2-ethenyl-1-methylpyridinium | C8 H10 N | 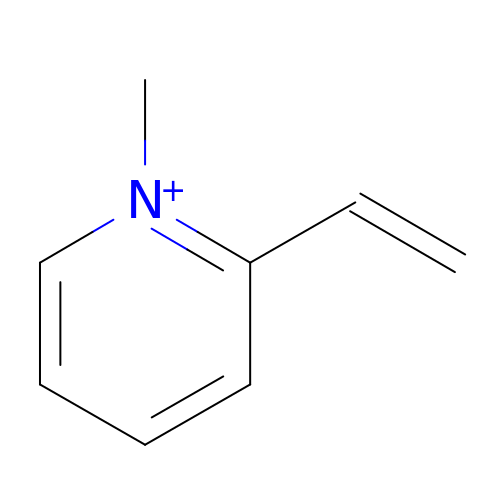DTJIKSRARSRPBU-UHFFFAOYSA-N> MPYIEKLELKGFKSYGNKKVVIPFSKGFTAIVGANGSGKSNIGDAILFVLGGLSAKAMRASRISDLIFAGSKNEPPAKYAE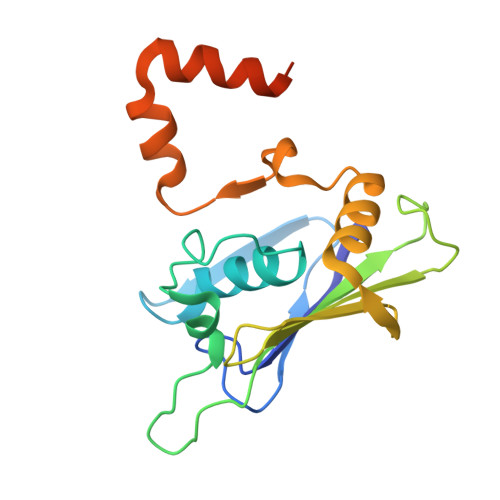VAIYFNNEDRGFPIDEDEVVIRRRVYPDGRSSYWLNGRRATRSEILDILTAAMISPDGYNIVLQGDITKFIKMSPLERRLLIDDISGIAEYDSKKEKALEE[(2~{S},5~{R})-1-[(2~{R},3~{S},4~{R},5~{R})-5-(6-aminopurin-9-yl)-3,4-bis(oxidanyl)oxolan-2-yl]-5-azaniumyl-6-oxidanyl-6-oxidanylidene-hexan-2-yl]-[(2~{R})-2-oxidanylpropyl]azanium 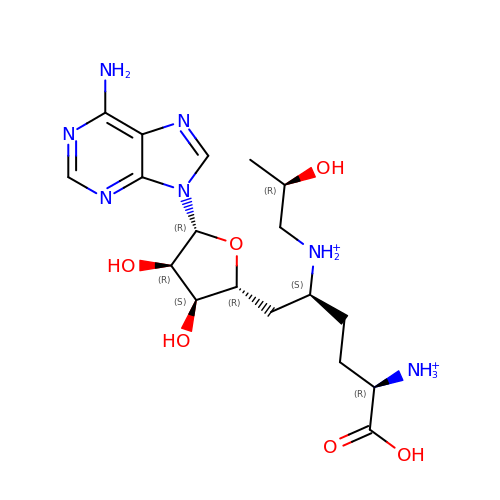| C18 H31 N7 O6 | OTZLYSCRIUWVSV-LZABMDAUSA-P> MSSLSRELVFLILQFLDEEKFKETVHKLEQESGFFFNMKYFEEKVHAGEWDEVEKYLSGFTKVDDNRYSMKIFFEIRKQKYLEALDRHDRAKAVDILVKDLKVFSTFNEEAYKEITQLLTLENFRENEQASKYGDTK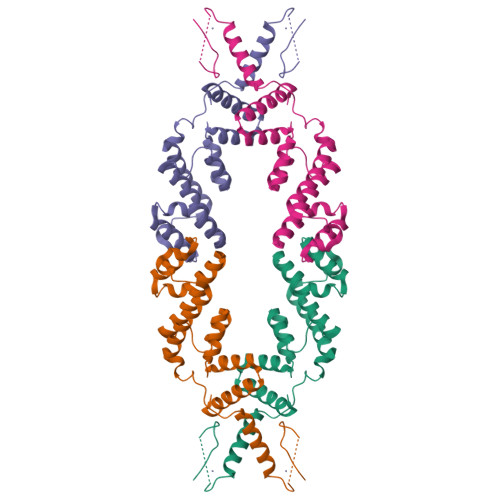SARSIMLIELKKLIEANPLFREKLVFPTLKASRLRTLINQSANWQHQLCKNPRPNPDAKTLFTDHTCTPPNG>[2x]MVTMEEIRKAQRAEGLATILAISTATPPNCVIQADYPDYYFKITNSEHMTELKEKFRRLCEKSMIRKRHMCLTEEILKA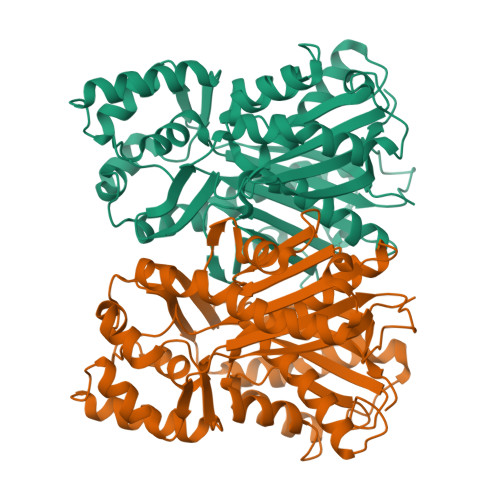NPNMCLHMGTSLNARQDISLVEVPKLGKEAATKAIKEWGQPKSKITHLIFCTSAGVDMPGADYQLTRLLGLSPEVKRMMIYQQGCYAGATVLRLAKDLTENNKGSRVLIVCSENTVPTFRGPSDTHIDSLVGQALFADGAAALIVGADPDASIERPLYHIVSASQTLLPDSDGAIEGHIREAGLTVHLKKDVPAFFSANIEKSLVDAFTPIGISDWNSIFWIAHPGGPAILDQVEEKLGLRKDKLKASRHVMSEFGNMSSACVLFILDEMRKTCLEEGKATTGEGLDWGVLFGFGPGLTVETVVLRSVPIEA> XSSDPL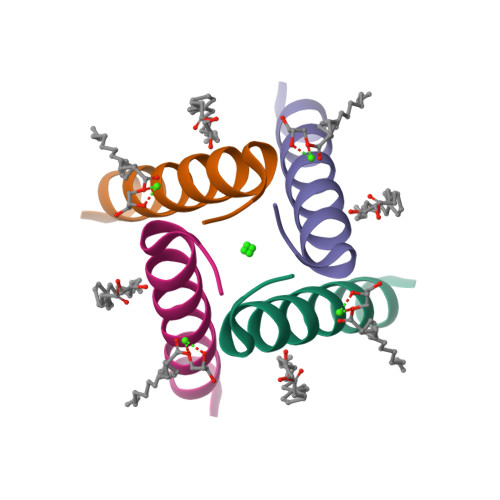VVAANIIGILHLILWILDRLX>[2x]MASDASVADSLDTLAAKLIEKAKDLRAGNSTTPQQHEALVGTLKQVQDAV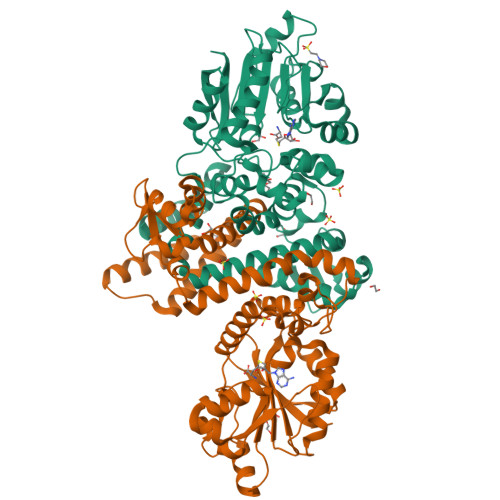YLPRDDLAAMQMGFVTAAAIRLLLHWKVFEKIPDTGSIRYEELATQVGGDVVIITRICWLLVATGFLVQEGSDRVAHTARTRPFAGVNPLRAWWLMGYDEYVPVLLAMPRYYDTYGIKEPTGRLHTIKAFTEGSPELTVGEIMSRHPERTANMLISMSAMASQYPHTGFYDFSWVAPKAAESATRPLIVDIGGAKGWTLQAICKETPEIPISRCVLQDLSGVIQMVQTVGDEDIRSAQLMAIDFHKEQPVQGALVYMIRRILRDFGDDECVSILQHVVAAMAPDSKLLIADTVTGNPPSWFPAMLDFFLSTIGGKERTEEEFRKITARAGLRITGIHYSDKAEFAMIVCEKAEHHHHHH>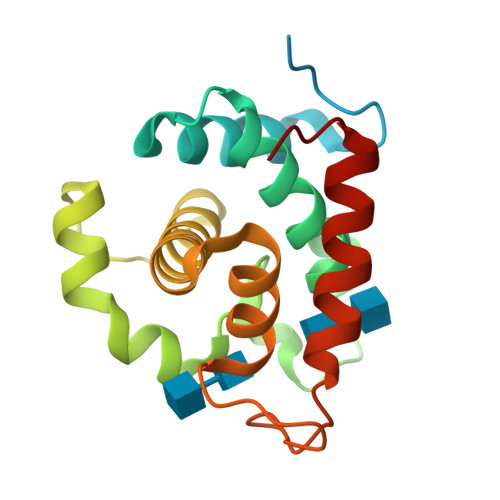[4x]MNHKVHHHHHHIEGRHMGTTPSDPPTNPPTTVTKPAEVPSRIWTYVMNADNAYGKGGDFALLLSAVIKKESYFGDGLSGSPSAGDGLMQVEPNTRNAYLSQFSAKYGHAYNHSSEQDQVYMGSLILNEKIVRFGSIYSGLLHYNGGDYWYPGATDSYGRPILADQYANTVYAQYKSYGGRYSR>MPGGKRGLVAPQNTFLENIVRRSSESSFLLGNAQIVDWPVVYSNDGFCKLSGYHRADVMQKSSTCSFMYGELTDKKTIEKVRQTFDNYESNCFEVLLYKKNRTPVWFYMQIAPIRNEHEKVVLFLCTFKDITLFKQPIEDDSTKGWTKFARLTRALTNSRSVLQQLTPMNKTEVVHKHSRLAEVLQLGSDILPQYKQEAPKTPPHIILHYCAFKTTWDWVILILTFYTAIMVPYNVSFKTKQNNIAWLVLDSVVDVIFLVDIVLNFHTTFVGPGGEVISDPKLIRMNYLKTWFVIDLLSCLPYDIINAFENVDEGISSLFSSLKVVRLLRLGRVARKLDHYLEYGAAVLVLLVCVFGLVAHWLACIWYSIGDYEVIDEVTNTIQIDSWLYQLALSIGTPYRYNTSAGIWEGGPSKDSLYVSSLYFTMTSLTTIGFGNIAPTTDVEKMFSVAMMMVGSLLYATIFGNVTTIFQQMYANTNRYHEMLNNVRDFLKLYQVPKGLSERVMDYIVSTWSMSKGIDTEKVLSICPKDMRADICVHLNRKVFNEHPAFRLASDGCLRALAVEFQTIHCAPGDLIYHAGESVDALCFVVSGSLEVIQDDEVVAILGKGDVFGDIFWKETTLAHACANVRALTYCDLHIIKREALLKVLDFYTAFANSFSRNLTLTCNLRKRIIFRKISDVKKEEEERLRQKNEVTLSIPVDHPVRKLFQKFKQQKELRNQGSTQGDPERNQLQVESRSLQNGASITGTSVVTVSQITPIQTSLAYVKTSESLKQNNRDAMELKPNGGADQKCLKVNSPIRMKNGNGKGWLRLKNNMGAHEEKKEDWNNVTKAESMGLLSEDPKSSDSENSVTKNPLRKTDSCDSGITKSDLRLDKAGEARSPLEHSPIQADAKHPFYPIPEQALQTTLQEVKHELKEDIQLLSCRMTALEKQVAEILKILSEKSVPQASSPKSQMPLQVPPQIPCQDIFSVSRPESPESDKDEIHF[4x]

Here, we report six structures with near-atomic resolution captured by cryo-EM, representing human Eag2 (hEag2) in closed, pre-open, open, and pore dilation but non-conducting states. We expressed full-length hEag2 fused with a green fluorescent protein (GFP) in HEK293T cells and characterized its electrophysiological properties and show that it is a voltage-activated delayed rectifier potassium channel with a half-activation membrane potential of −10.0 ± 3.5 mV. The channel has a three-layer architecture: the upper extracellular turret, transmembrane domains, and intracellular domains occupying 3D space with a size of 130 Å × 130 Å × 130 Å. The tetrameric hEag2 apparatus adopts noncanonical non-domain-swapped VSDs, with distinct pore domain configurations.

Six distinct configurations captured for hEag2 are primarily based on the pore dilation and ion distribution. The overall Cα atoms and the side chain of the two closed states are almost identical, while the differences are density peaks of the water molecule and potassium ion in S0, indicating that the water and potassium in S0 layer are dynamic in the closed states. For hEag2, in a closed state, the four pore-lining S6 helices form a bundle-crossing in the middle of the membrane right below the ion selectivity filter with two layers of hydroxyphenyl or phenyl residue, Y460s and F464s, forming the hydrophobic constriction sites through intrachain and interchain π–π interaction to prevent hydrated/dehydrated potassium ion flow. Below the hydrophobic constriction sites are hydrophilic constriction sites through intrachain and interchain electrostatic interaction of Q472s and T468s. The hydrophilic constriction sites together with the hydrophobic ones form a long channel gate. In the closed states and pre-open state 1, a strong and unambiguous density peak is located between the hydrophobic and hydrophilic constriction sites. The density is more likely to be a dehydrated potassium ion, and we name it site 6 or S6 as the seventh potassium ion selectivity site. If our closed states represent the deep closed state, we suspect that the voltage may act on both S4–S5 linkers and constricted sites for the hEag2 channel to sense the electromechanical force. However, there may exist a deep closed state (for example under −70 mV membrane potential condition), and our closed structures may still present a pre-open closed state.> GHMQIGWRREGIKYRRNELFLDVLESVNLLMSPQGQVLSAHVSGRVVMKSYLSGMPECKFGMNDKIVIEKQGKGTADETSKSGKQ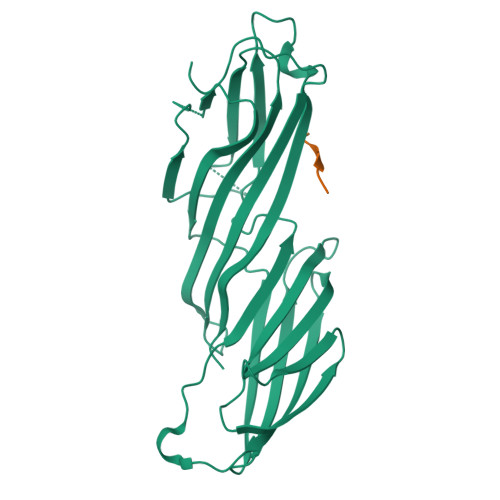SIAIDDCTFHQCVRLSKFDSERSISFIPPDGEFELMRYRTTKDIILPFRVIPLVREVGRTKLEVKVVIKSNFKPSLLAQKIEVRIPTPLNTSGVQVICMKGKAKYKASENAIVWKIKRMAGMKESQISAEIELLPTNDKKKWARPPISMNFEVPFAPSGLKVRYLKVFEPKLNYSDHDVIKWVRYIGRSGIYETRC;> LYCYEQLNDSSEEEDEID>[2x]DSNFPLPDLCSWEEAQLSSQLYRNKQLQDTLVQKEEELARLHEENNHLRQYLNSALVKCEEEKAKKELSSDEFSKAYGKFRKGKR

Geminin coiled-coil domain-containing protein 1, GemC1, is a member of the Geminin superfamily. The three members of this family, Geminin, Idas and GemC1, all share a conserved coiled-coil domain. GemC1 has been identified as a Geminin homologue, and is also implicated in DNA replication but at a later stage than Geminin. GemC1 has been shown to mediate TopBP1- and Cdk2-dependent recruitment of Cdc45 onto replication origins, enabling pre-initiation complex formation and initiation of DNA replication.

To better understand this family of proteins, the crystal structure of a GemC1 coiled-coil domain variant engineered for better solubility was determined to 2.2 Å resolution. In particular, at the C-terminal end of the coiled coil, residues Leu119, Val120, Leu123, Ala127, Leu130 and Leu131 constitute a hydrophobic patch. We thus decided to mutate residues Leu123 and Leu130 to glutamates to increase the solubility. Our mutations yielded the construct tGemC1L123,130E, which allowed the expression of highly soluble protein (>2 mM). Residues 71–129 and 70–124 are in α-helical conformation in each chain. The two mutated leucine residues are indeed pointing to the solvent, as expected from our sequence analysis and in contrast to the other predictions discussed above. Based on our structural data, we conclude that the change of the hydrophobic solvent-exposed Leu123 and Leu130 to hydrophilic glutamate residues improved solubility without affecting the global structure. Analysis of the structure using the SOCKET software shows that the coiled-coil region extends from residues 73 to 115 and spans six heptads (technically speaking, one residue of a seventh heptad is present). Analysis of the coiled-coil parameters by the program CCCP shows that the GemC1 coiled coil has an ω0 angle of −4.1° per residue, suggesting a relatively tight left-handed superhelix compared with the Geminin homodimer (ω0 = −3.9° per residue) and Idas–Geminin (ω0 = −3.7° per residue). The superhelical radius (the distance from the superhelix axis to the helical axis of the chains) is longer in GemC1 at 5.1 Å compared with 4.7 Å for both Geminin and Idas–Geminin.(3-PYRAZOL-1-YLPHENYL)METHANAMINE | C10 H11 N3 | 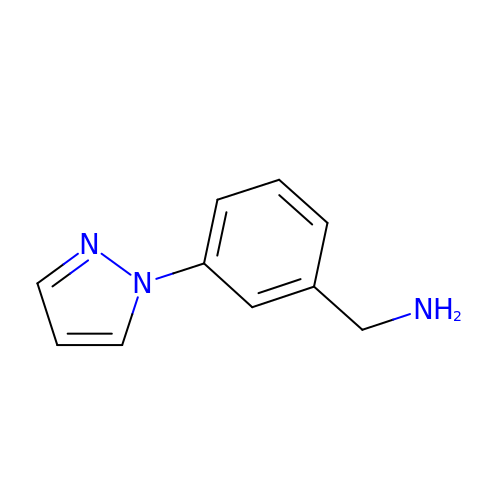YWZKZHCZKIKAAC-UHFFFAOYSA-N>[2x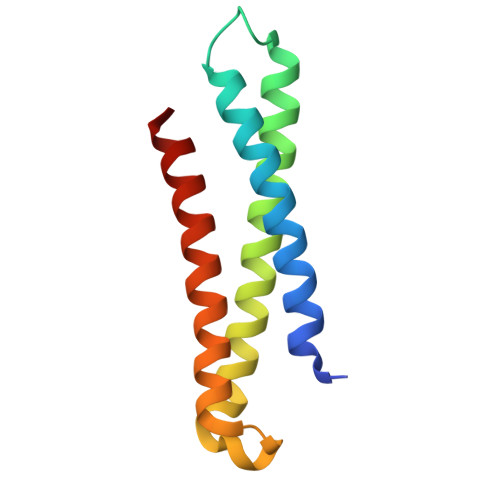]MSMEDPFFVVKGEVQKAVNTAQGLFQRWTELLQGPSAATREEIDWTTNELRNNLRSIEWDLEDLDETISIVEANPRKFNLDATELSIRKAFITSTRQIVRDMKDQMSASS N-{3-[(1S)-2-(3-{(Z)-[amino(thiophen-2-yl)methylidene]amino}phenoxy)-1-hydroxyethyl]phenyl}thiophene-2-carboximidamide | C24 H22 N4 O2 S2 | 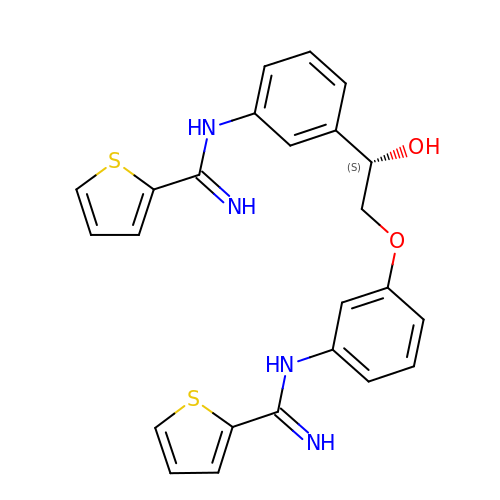ZCTCFQXRJWOQIL-HXUWFJFHSA-N Disopyramide | C21 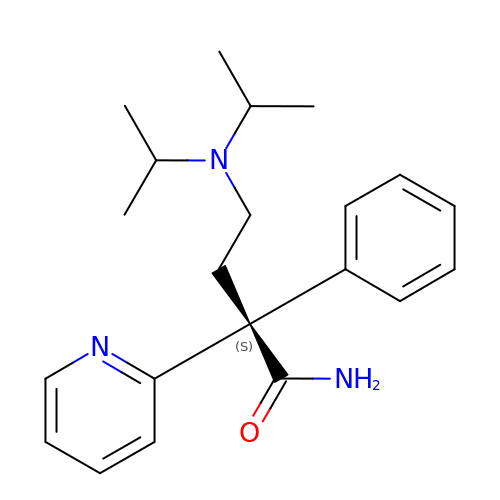H29 N3 O | UVTNFZQICZKOEM-NRFANRHFSA-N>[2x]MASWSHPQFEKGAVTSLYKKAGFSDKYYRSAYMNVDLNAVASNFKVFSTLHPNKTVMAVVK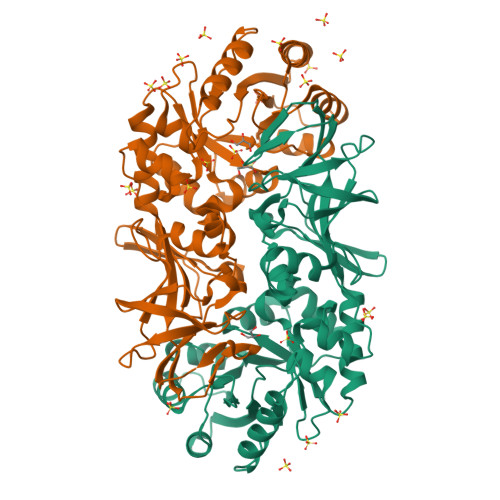ANAYGLGSVKVARHLMENGATFFAVATLDEAIELRMHGITAKILVLGVLPAKDIDKAIQHRVALTVPSKQWLKEAIKNISGEQEKKLWLHIKLDTGMGRLGIKDTNTYQEVIEIIQQYEQLVFEGVFTHFACADEPGDMTTEQYQRFKDMVNEAIKPEYIHCQNSAGSLLMDCQFCNAIRPGISLYGYYPSEYVQQKVKVHLKPSVQLIANVVQTKTLQAGESVSYGATYTATDPTTIALLPIGYADGYLRIMQGSFVNVNGHQCEVIGRVCMDQTIVKVPDQVKAGDSVILIDNHRESPQSVEVVAEKQHTINYEVLCNLSRRLPRIYHDGDQRFVTNELLK1-pyrrolo[1,2-a]quinoxalin-4-ylnaphthalen-2-ol | C21 H14 N2 O | 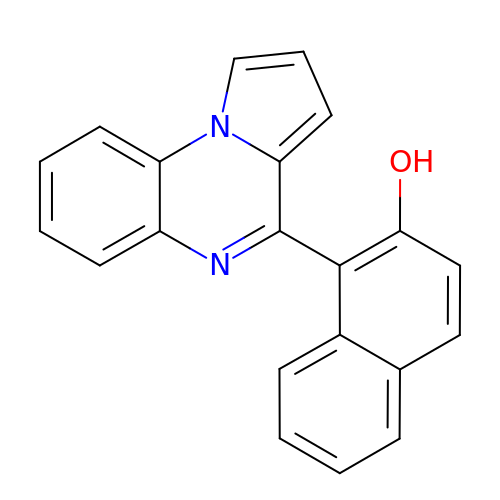IESKGGHNIDBTKX-UHFFFAOYSA-N The capsaicin- and heat-activated receptor, TRPV1, has served as a model for deciphering lipid modulation, which is relevant to understanding how pro-algesic agents enhance channel activity in the setting of inflammatory pain. Identification of a pocket within the TRPV1 transmembrane core has provided initial clues as to how phosphoinositide lipids bind to and regulate the channel. Here we show that this regulatory pocket in rat TRPV1 can accommodate diverse lipid species, including the inflammatory lipid lysophosphatidic acid, whose actions are determined by their specific modes of binding. We captured several states of TRPV1 ranging from channels in which the VBP is empty to those bearing different bioactive lipids, including distinct phosphoinositide species, brominated phosphoinositide analogs and a pro-algesic lipid, lysophosphatidic acid (LPA). Together, our data show how the VBP accommodates a range of bioactive lipids and how occupancy of the site corresponds to the structural status of the pore.

We therefore obtained cryo-EM data for samples in which diC8-PIP2 was provided to the empty-pocket TRPV1 preparation. Using focused classification, we were able to identify two key states, one corresponding to a closed state (3.0 Å) and the other having a dilated selectivity filter (3.6 Å). In the dilated state, diC8-PIP2 sits higher up in the vanilloid pocket such that the inositol headgroup sits above Y511, which is reorientated toward the pocket. Moreover, Y671 adopts an α-helical conformation and M682 and is oriented toward the pore axis. These features are hallmarks of a channel in which the resident PI lipid has been displaced (that is, the pocket is empty or occupied by a vanilloid agonist). However, there are some differences between the diC8-PIP2 dilated state and a typical vanilloid agonist-bound structure. Most notably, in the diC8-PIP2 dilated state the angle of the S6 helix is more dramatically tilted such that the voltage sensor-like domain (S1–S4, VSLD) is pivoted outward away from the central axis, and the upper region of the ion permeation pathway, including the selectivity filter, is expanded and stabilized by cholesterol and another membrane lipid (probably 1,2-dioleoyl-sn-glycero-3-phosphocholine (DOPC)). At the same time, pivoting of the S6 helix makes the new restriction site formed by M682 narrower. Thus, this dilated structure is consistent with the functional effects of diC8-PIP2, which enhances capsaicin sensitivity, but by itself activates the channel only at highly depolarized states (for example, +150 mV membrane potential)8,9. In this case, one ligand can bind to the same pocket but with its inositol headgroup located in two distinct positions associated with closed or dilated pore states.

>[4x]MGSRLYDRRSIFDAVAQSNCQELESLLPFLQRSKKRLTDSEFKDPETGKTCLLKAMLNLHNGQNDTIALLLDVARKTDSLKQFVNASYTDSYYKGQTALHIAIERRNMTLVTLLVENGADVQAAANGDFFKKTKGRPGFYFGELPLSLAACTNQLAIVKFLLQNSWQPADISARDSVGNTVLHALVEVADNTVDNTKFVTSMYNEILILGAKLHPTLKLEEITNRKGLTPLALAASSGKIGVLAYILQREIHEPECRHLSRKFTEWAYGPVHSSLYDLSCIDTCEKNSVLEVIAYSSSETPNRHDMLLVEPLNRLLQDKWDRFVKRIFYFNFFVYCLYMIIFTAAAYYRPVEGLPPYKLKNTVGDYFRVTGEILSVSGGVYFFFRGIQYFLQRRPSLKSLFVDSYSEILFFVQSLFMLVSVVLYFSQRKEYVASMVFSLAMGWTNMLYYTRGFQQMGIYAVMIEKMILRDLCRFMFVYLVFLFGFSTAVVTLIEDGKYNSLYSTCLELFKFTIGMGDLEFTENYDFKAVFIILLLAYVILTYILLLNMLIALMGETVNKIAQESKNIWKLQRAITILDTEKSFLKCMRKAFRSGKLLQVGFTPDGKDDYRWCFRVDEVNWTTWNTNVGIINEDPG>[3x]AAYSQGGGKKKVCYYYDGDIGNYYYGQGHPMKPHRIRMTHNLLLNYGLYRKMEIYRPHKATAEEMTKYHSDEYIKFLRSIRPDNMSEYSKQMQRFNVGEDCPVFDGLFEFCQLSTGGSVAGAVKLNRQQTDMAVNWAGGLHHAKKSEASGFCYVNDIVLAILELLKYHQRVLYIDIDIHHGDGVEEAFYTTDRVMTVSFHKYGEYFPGTGDLRDIGAGKGKYYAVNFPMRDGIDDESYGQIFKPIISKVMEMYQPSAVVLQCGADSLSGDRLGCFNLTVKGHAKCVEVVKTFNLPLLMLGGGGYTIRNVARCWTYETAVALDCEIPNELPYNDYFEYFGPDFKLHISPSNMTNQNTPEYMEKIKQRLFENLRMLPHAPGVQMQAI;>XNPKQKWG[3x]

To address this challenge, we develop a computational “anchor extension” methodology for targeting protein interfaces by extending a peptide chain around a non-canonical amino acid residue anchor. To test our approach using a well characterized model system, we design cyclic peptides that inhibit histone deacetylases 2 and 6 (HDAC2 and HDAC6) with enhanced potency compared to the original anchor (IC50 values of 9.1 and 4.4 nM for the best binders compared to 5.4 and 0.6 µM for the anchor, respectively). SHA can coordinate to the zinc ion in the active site of HDACs. In all the crystal structures we obtained, the thiol functional group of SHA coordinates the catalytic Zn2+ ion with a Zn2+– S separation of 2.3 Å in a distorted tetrahedral geometry reminiscent of that observed for the inhibitor Largazole.

Our first computational method (design method 1) started with docking structured cyclic-peptide scaffolds onto SHA and re-designing the residues in the interface to improve binding. Tens of thousands of conformers were generated for each of the 100 peptides, their energies were evaluated, and those designs for which the designed target structure had the lowest energy were selected for downstream analysis. From the previous pool, five peptides with the greatest in silico predicted affinities were tested for HDAC2 inhibition in vitro, the best of which (des1.1.0) demonstrated an IC50 value of 289 nM. The crystal structure of this design in complex with HDAC2 revealed two distinct binding modes and peptide conformations in the three protein chains of the asymmetric unit, suggesting flexibility of the peptide as well as presence of iso-energetic binding conformations. In two of the protein chains of the asymmetric unit (chains B and C), the peptide conformation was very similar to the design model, but the observed binding mode to HDAC2 differed from that of the design model. This binding orientation interacts with several water molecules through backbone-mediated hydrogen bonds. Rosetta-guided mutational scanning successfully stabilized the binding mode observed in the crystal structure (confirmed by structures of variants Lys4→Glu and Pro3→hydroxy-Pro) but failed to significantly improve affinity or selectivity.>[3x]MHHHHHHGAQPARSANDTVVVGSIIFTEGIIVANMVAEMIEAHTDLKVVRKLNLGGYNVNFEAIKRGGANNGIDIYVEYTGHGLVDILGFPATTDPEGAYETVKKEYKRKWNIVWLKPLGFNNTYTLTVKDELAKQYNLKTFSDLAKISDKLILGATMWFLEGPDGYPGLQKLYNFKFKHTKSMDMGIRYTAID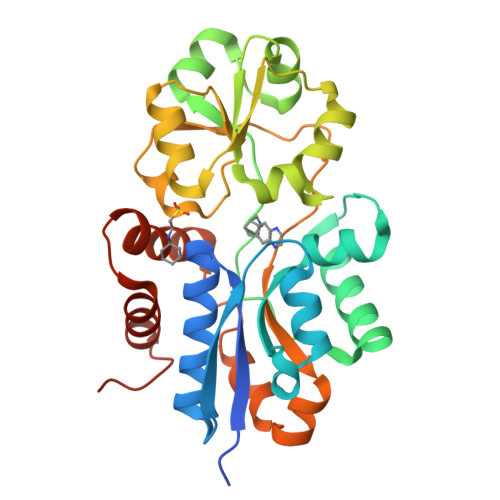NNEVQVIDAWATDGLLVSHKLKILEDDKAFFPPYYAAPIIRQDVLDKHPELKDVLNKLANQISLEEMQKLNYKVDGEGQDPAKVAKEFLKEKGLILQVD>GEFEAVPRMPMIWLDLKEAGDFHFQPAVKKFVLKNYGENPEAYNEELKKLELLRQNAVRVPRDFEGCSVLRKYLGQLHYLQSRVPMGSGQEAAVPVTWTEIFSGKSVAHEDIKYEQACILYNLGALHSMLGAMDKRVSEEGMKVSCTHFQCAAGAFAYLREHFPQAYSVDMSRQILTLNVNLMLGQAQECLLEKSMLDNRKSFLVARISAQVVDYYKEACRALENPDTASLLGRIQKDWKKLVQMKIYYFAAVAHLHMGKQAEEQQKFGERVAYFQSALDKLNEAIKLAKGQPDT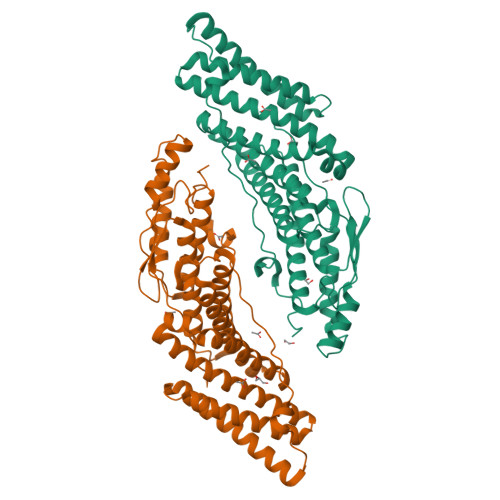VQDALRFTMDVIGGKYNSAKKDNDFIYHEAVPALDTLQPVKGAPLVKPLPVNPTDPAVTGPDIFAKLV[2x]> MIKLFSLKQQ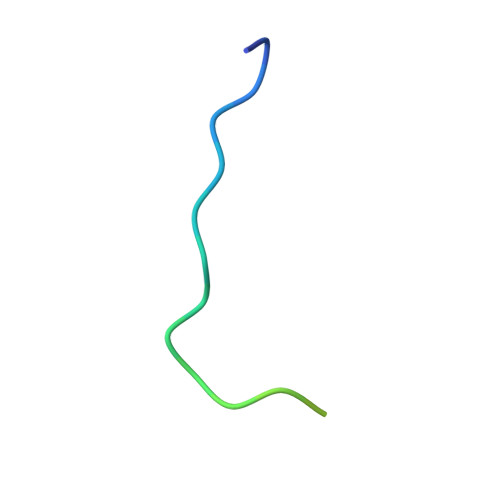KKEEESAGGTKGSSKK>PIIDQGPLPTLTDGDKKAINKIWPKIYKEYEQYSLNILLRFLKCFPQAQASFPKFSTKKSNLEQDPEVKHQAVVIFNKVNEIINSMDNQEEIIKSLKDLSQKHKTVFKVDSIWFKEL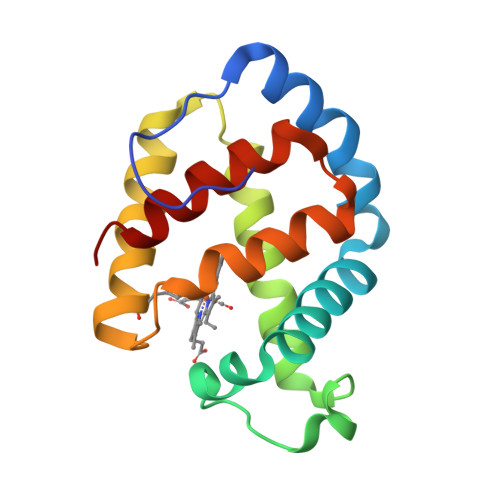SSIFVSTIDGGAEFEKLFSIICILLRSAY[4x]>[2x]GMGQRSDSDHVMAEATTDKRQGHTRGRTGNDRRTQIIKVATELFREKGYYATS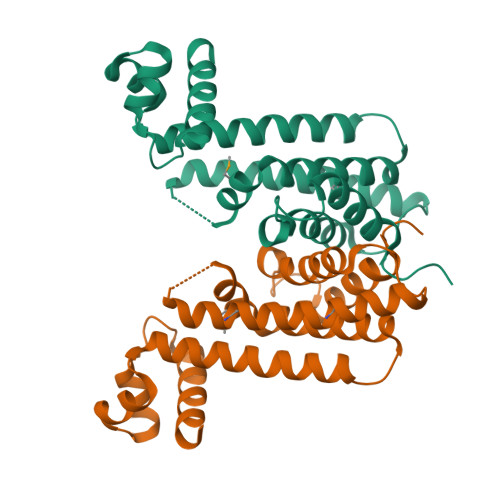LDDIADRIGFTKPAIYYYFKSKEDVLFAIVNSIVDEALERFHAIAAGPGSPGERIHALLVEHTRTILRNLDANTLFYNERGLLSPEREREMRKREREYTEIMQRLYAEGVATGELLDVDPTVATATLLGAAIWTYRWYDPEGRLSADEVVEQITRLLLNGYRRPA> MVECSGNLFTQRTGTITSPDYPNPYPK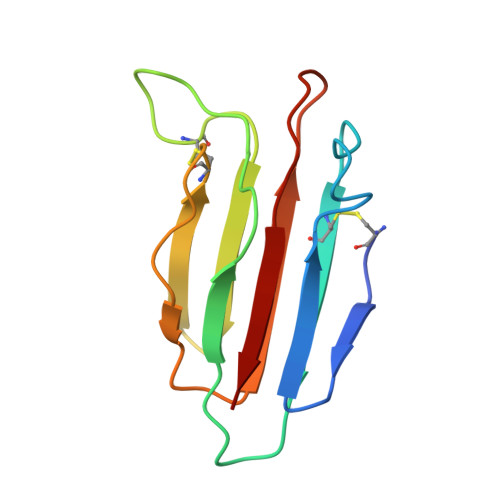SSECSYTIDLEEGFMVTLQFEDIFDIEDHPEVPCPYDYIKIKAGSKVWGPFCGEKSPEPISTQSHSIQILFRSDNSGENRGWRLSYRA> MAEPLLVVG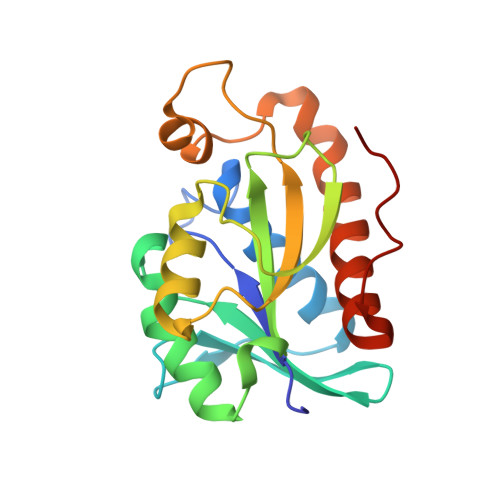LGNPGANYARTRHNLGFVVADLLAARLGAKFKAHKRSGAEVATGRSAGRSLVLAKPRCYMNESGRQIGPLAKFYSVAPANIIVIHDDLDLEFGRIRLKIGGGEGGHNGLRSVVAALGTKDFQRVRIGIGRPPGRKDPAAFVLENFTPAERAEVPTICEQAADATELLIEQGMEPAQNRVHAW>AKKIGLFYGTQTGKTESVAEIIRDEFGNDVVTLHDVSQAEVTDLNDYQYLIIGCPTENIGELQSDWEGLYSELDDVDFNGKLVAYFGTGDQIG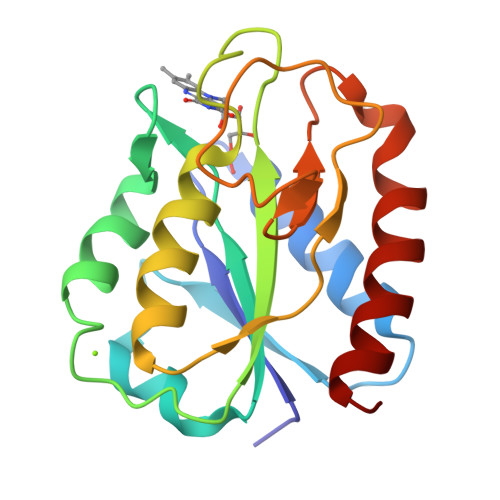YADNFQDAIGILEEKISQRGGKTVGYWSTDGYDFNDSKALRNGKFVGLALDEDNQSDLTDDRIKSWVAQLKSEFGL[2x]> MVMTELILHHYATSPFSEKARLILGYKDQPWKSVTVPVILPKPDVMPLTGGYRRTPFLQIGADIYCDTALIAQVLESIHPVPTLYPADRAAAAFAMAQWADTTLFWAAASFVGQPEGFKSLMAGLPEDFVKAFVEDRKAMRAGGTGLRTPLPEAVATLQVFLAQLERQFATGEHIFLFGEQPTIADFSVYHALWFIRRAT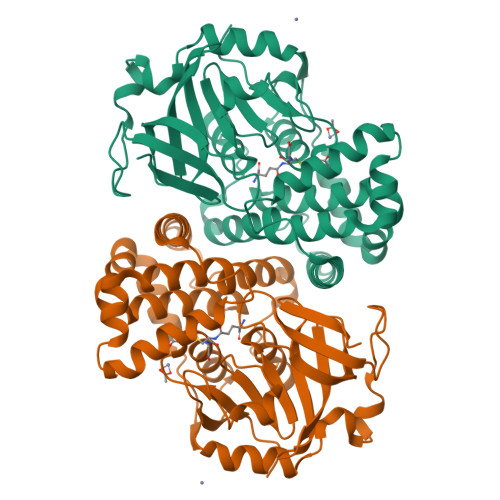AVAGILDAHPEVVAWMHRMAGFGHAQAQPMTPAEALAIARAATPRALTDAGAGADFDARYGLPKGTRVTVAATDYAVDPVEGDLVVSTRDAVGVLREDPRVGQVVVHFPRVGYAVRKVEPAGAENLYFQ>MISILHYGYSFIMLLGALYFYLLSKDPKGVPASEYLIAMVIPLWSGAAYLSIALGQGLFQYDDTTIYYARYIDWVISTPLLLAALALTAMFGGKKNLTLLFSLVALDVFMIITGFVADLSIGTTKYIWYSLGVIALIIILVITFGPLRRIALSNGTRLARHYTRVA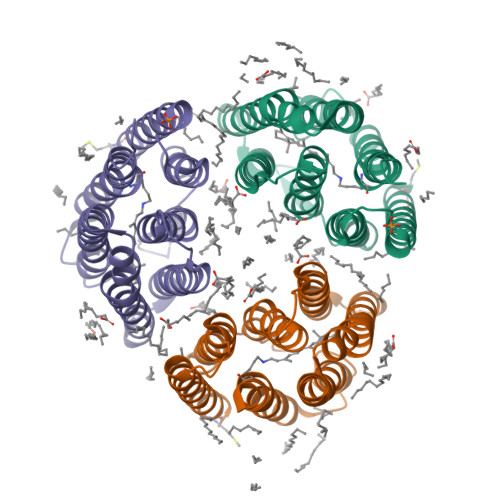IYLSALWVCYPTAWLLGPSGLGLAQELTEVLVFIILPIFSKVGFSIVDLHGLRKLHQSSYVHN[3x]> HSDAQVLVLLDVTPDQSMVDEG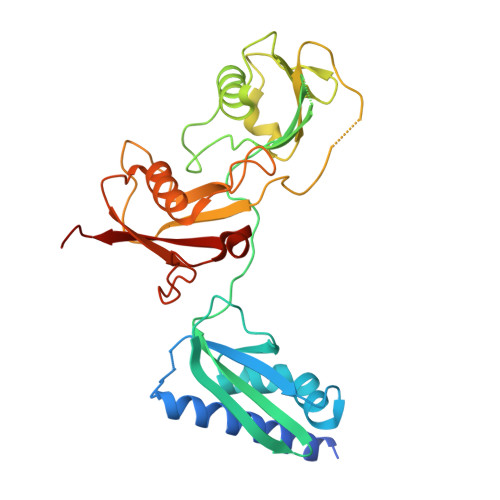VAREVINRIQKLRKKRNLVPTDEITVYYRSHPEGDYLDTVIKEHTDFIFATIKAALKPYPVPTSKEVLIQETTQLKGSELEITLVRGGLCERVGPACSYVNLKVCVNGTEQDGVLLLENPKGDNTLNLTGLVDAVSCIFGLKNSKLTVFNGKTELINKTDLLSLSGKTLHVTTGSAPALINSPDALLCQYINLQLVNAKPQECQKGTVGTLLMENPVGQNGLTYHGLLHETAKVFGLRSRRLKLFLDEAETQEITKDISMKNLNMKTVYVSVIPTTAEC>MSFDDLHKATERAVIQAVDQICDDFEVTPEKLDELTAYFIEQMEKGLAPPKEGHTLASDKGLPMIPAFVTGSPNGTERGVLLAADLGGTNFRICSVNLHGDHTFSMEQMKSKIPDDLLDDENVTSDDLFGFLARRTLAFMKKYHPDELAKGKDAKPMKLGFTFSYPVDQTSLNSGTLIRWTKGFRIADTVGKDVVQLYQEQLSAQGMPMIKVVALTNDTVGTYLSHCYTSDNTDSMTSGEISEPVIGCIFGTGTNGCYMEEINKITKLPQELRDKLIKEGKTHMIINVEWGSFDNELKHLPTTKYDVVIDQKLSTNPGFHLFEKRVSGMFLGEVLRNILVDLHSQGLLLQQYRSKEQLPRHLTTPFQ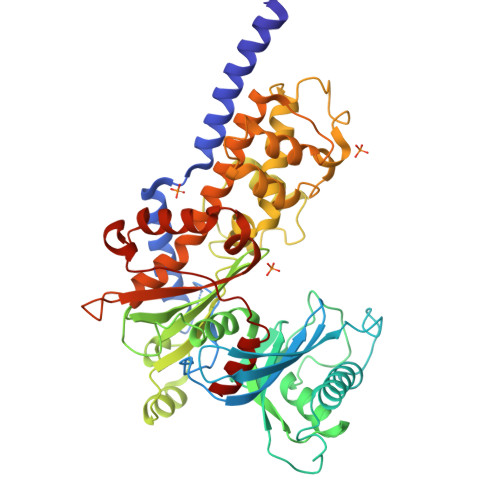LSSEVLSHIEIDDSTGLRETELSLLQSLRLPTTPTERVQIQKLVRAISRRSAYLAAVPLAAILIKTNALNKRYHGEVEIGCDGSVVEYYPGFRSMLRHALALSPLGAEGERKVHLKIAKDGSGVGAALCALVA[6x]SAA1.1 is an acute phase protein that becomes strongly upregulated during inflammation. Chronic inflammatory conditions, such as tuberculosis, leprosy and rheumatoid arthritis, are risk factors for the development of systemic AA amyloidosis. We report three cryo-EM structures of SAA1.1-derived amyloid fibrils: one that was extracted from the diseased murine tissue and two that were formed from murine SAA1.1 protein in vitro. In vitro and ex vivo fibrils possess parallel cross-β sheets but differ in their overall topologies and fibril protein folds.

In vitro formed fibrils are also polymorphic and contain one major fibril morphology (morphology i). This fibril corresponds to 75% of the fibrils present in solution and is considerably thinner than the other analyzed fibril morphology, termed here morphology ii. Cryo-EM reconstructions achieved spatial resolutions of 2.73 Å for morphology i and 2.95 Å for morphology ii. Morphology i is polar and presents a pseudo 21-screw symmetry. A single PF consists of two structurally equal stacks of fibril proteins that are arranged such that residues Gly1 and Phe2 from one stack interact with residues Asp22-Lys24 in the other stack. The Gly1 α-amino group is in the vicinity of the Asp22 side chain, while Phe2 inserts into a small pocket formed by Asp22-Lys24 main chain and side chain atoms. The PF encloses a large internal cavity that appears water filled as it is lined with polar (Thr21) and charged (Gly1, Asp22) amino acid residues. The ordered core of the in vitro fibrils is considerably smaller and formed by residues 1-37. The in vitro fibril contains seven β-strands (β1 to β7) at residues Phe2-Ile6, Glu8-Gln11, Asp15-Met16, Arg18-Thr21, Met23-Lys24, Ala26-Asp30, and Asp32-His36. Residues 1–37 form two partially overlapping arches (Gly1-Thr21 and Gly12-His36), reminiscent of the ex vivo fibril.

>GFFSFIGEAFQGAGDMWRAYTDMKEAGWKDGDKYFHARGNYDAAQRGPGGVWAAEKISDARESFQEFFGRGHEDTMADQEANRHGRSGKDPNYYRPPGLPAKY[12x]The cholesterol-dependent cytolysin (CDC), pneumolysin is a virulence factor of the human pathogen Streptococcus pneumoniae (pneumococcus)2, the leading cause of bacterial pneumonia and a major agent of meningitis and septicaemia as well as debilitating diseases such as otitis media, septic arthritis, keratitis and sinusitis. A central feature of the toxin is the formation of transmembrane pores in cholesterol-containing membranes, which lyse or disrupt cell functioning, depending on the concentration. Pneumolysin and other CDCs bind to mammalian membranes through a tryptophan-rich loop and a threonine-leucine pair within a membrane-binding domain at the base of the toxin. Once bound to the membrane, monomers then oligomerise to form a pre-pore complex that subsequently undergoes a complex set of structural transitions to form a transmembrane pore, typically comprising 30–50 subunits.

Full-length pneumolysin and a truncated form comprising the membrane-binding domain (domain 4) were produced by expression in E. coli and purified by affinity and gel filtration chromatography. Crystal of the membrane-binding domain were grown at room temperature and contained two molecules in the asymmetric unit. By contrast, the loop is partially folded back in the structure of domain 4 alone, and fully bent back against the body of domain 4 in the previously determined structure of perfringolysin O12. Together the structures are consistent with previous suggestion that the loop springs outwards and downwards when the toxin binds to the membrane of a mammalian cell. In the crystal structure, Glu434 not only forms a salt bridge with Arg399 but also interacts with Arg437 that in turn forms part of the binding interface by packing against the adjacent monomer. Interestingly, these interactions are only possible when the tryptophan-rich loop is flipped outwards in the putative membrane-binding conformation. When the loop is folded back, as in the domain 4 structure or in the structure of perfringolysin O, Glu434 no longer contacts Arg399 or Arg437. In solution, Glu434 does not contact Arg437, so is unable to contribute towards monomer-monomer packing.

>RNGDLLLDHSGAYVAQYYITWNELSYDHQGKEVLTPKAWDRNGQDLTAHFTTSIPLKGNVRNLSVKIRECTGLAWEWWRTVYEKTDLPLVRKRTISIWGTTLYPQVEDKVEND[2x]> GPPGGVTEGIIARVA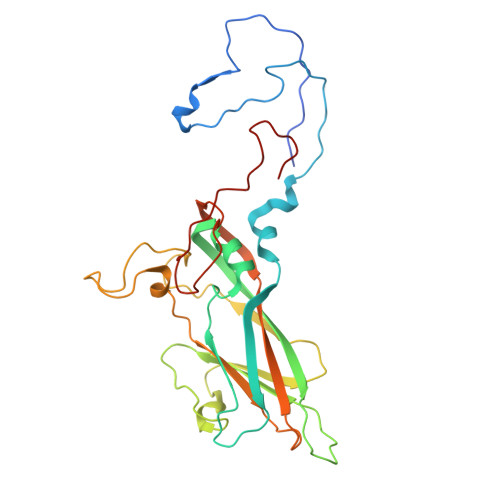DTVGSGPVNSESIPALTAAETGHTSQVVPSDTMQTRHVKNYHSRSESTVENFLCRSACVFYTTYKNHDSDGDNFAYWVINARQVAQLRRKLEMFTYARFDLELTFVITSTQEQSTTQGQDTPVLTHQIMYVPPGGPVPTKVNSYSWQTSTNPSVFWTEGNAPPRMSIPFIGIGNAYSMFYDGWARFDKQGTYGISTLNSMGTLYMRHVNGGGPGPIVSTVRIYFKPKHVKTWVPRPPRLCQYKKAGNVNFIPTSVTEGRTDITTMKTT>GAMTIRHQGQQYRPRMAFLQKIEALVKDMQNPETGVRMHNQRVLVTSVPHAMTGGDVLQWITQRLWISNLEAQNLGNFIVKYGYIYPLQDPKNLILKPDSSLYRFQTPYFWPTQQWPAEDTDYAIYLAKRNIKKKGILEEYEKENYDFLNKKINYKWDFVIMQAKEQYRTGKERNKADRYALDCQEKAYWLVHRSPPGMNNVLDYGLDRVTNPNEVKKQTVTAVRKEIMYYQQALMRSTVKSSVSLGGIVKYSEQFSSNDAIMSGCLPSNPWITDDTQFWDLNAKLVEIPTKMRVERWAFNFSELIRDPKGRQSFQYFLKKEFSGENLGFWEACEDLKYGDQSKVKEKAEEIYKLFLAPGARRWINIDGKTMDITVKGLRHPHRYVLDAAQTHIYMLMKKDSYARYLKSPIYKEMLAKAIEPQE[2x];>GMATDGLHENETLASLKSEAESLKGKLEEERAKLHDVELHQVAERVEALGQFVMKTRRTLKGHGNKVLCMDWCKDKRRIVSSSQDGKVIVWDSFTTNKEHAVTMPCTWVMACAYAPSGCAIACGGLDNKCSVYPLTFDKNENMAAKKKSVAMHTNYLSACSFTNSDMQILTASGDGTCALWDVESGQLLQSFHGHGADVLCLDLAPSETGNTFVSGGCDK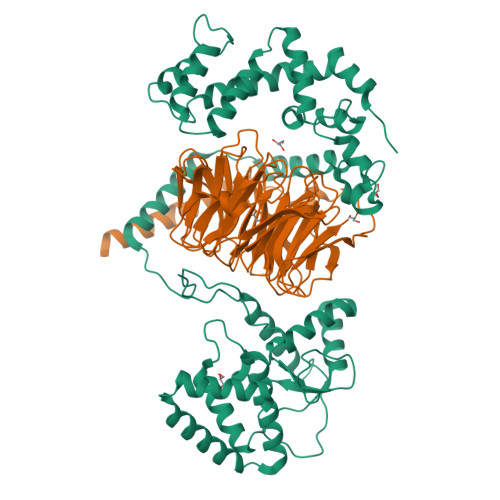KAMVWDMRSGQCVQAFETHESDVNSVRYYPSGDAFASGSDDATCRLYDLRADREVAIYSKESIIFGASSVDFSLSGRLLFAGYNDYTINVWDVLKGSRVSILFGHENRVSTLRVSPDGTAFCSGSWDHTLRVWA[2x]> MELRHTPARDLDKFIEDHLLPNTCFRTQVKEAIDIVCRFLKERCFQGTADPVRVSKVVKGGSSGKGTTLRGRSDADLVVFLTKLTSFEDQLRRRGEFIQEIRRQLEACQREQKFKVTFEVQSPRRENPRALSFVLSSPQLQQEVEFDVLPAFDALGQWTPGYKPNPEIYVQLIKECKSRGKEGEFSTCFTELQRDFLRNRPTKLKSLIRLVKHWYQTCKKTHGNKLPPQYALELLTVYAWEQGSRKTDFSTAQGFQT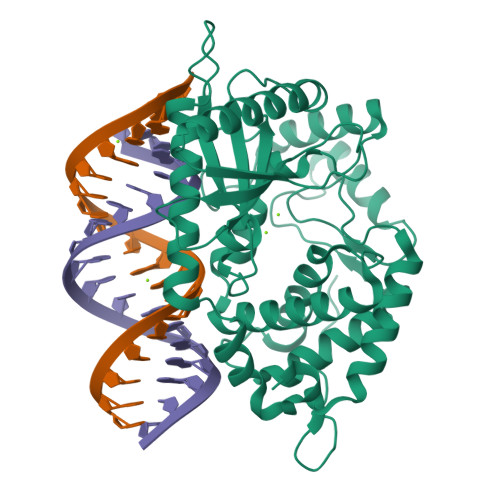VLELVLKHQKLCIFWEAYYDFTNPVVGRCMLQQLKKPRPVILDPADPTGNVGGGDTHSWQRLAQEARVWLGYPCCKNLDGSLVGAWTMLQKIGSHHHHHH>[4x]MTNSNHKNLTTNQGVPVGDNQNSRTAGHRGPSFLDDYHLIEKLAHFDRERIPERVVHARGAGAYGVFEVENSMEKHTRAAFLSEEGKQTDVFVRFSTVIHPKGSPETLRDPRGFAVKFYTEEGNYDLVGNNLPIFFIRDALKFPDMVHSLKPDPVTNIQDP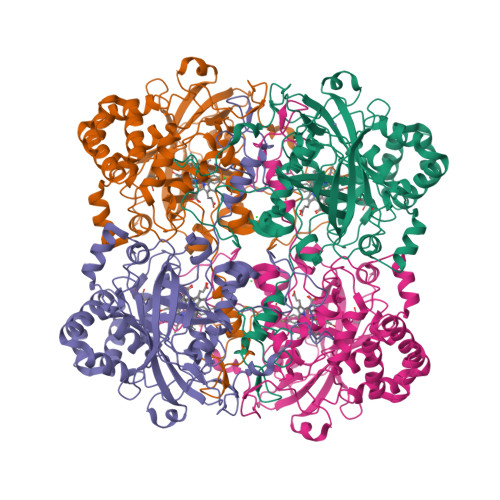DRYWDFMTLTPESTHMLTWLFSDEGIPANYAEMRGSGVHTFRWVNKYGETKYVKYHWRPSEGIRNLSMEEAAEIQANDFQHATRDLYDRIEKGNYPAWDLYVQLMPLSDYDELDYDPCDPTKTWSEEDYPLQKVGRMTLNRNPENFFAETEQAAFTPSALVPGIEASEDKLLQGRLFSYPDTQRHRLGANYMRIPVNCPYAPVHNNQQDGFMTTTRPSGHINYEPNRYDDQPKENPHYKESEPVLHGDRMVRQKIEKPNDFKQAGEKYRSYSEEEKQALIKNLTADLKGVNEKTKLLAICNFYRADEDYGQRLADSLGVDIRSYLQGSMK> SSQIRQNYSTEVEAAVNRLVNLYLRASYTYLSLGFYFDRDDVALEGVCHFFRELAEEKREGAERLLKMQNQRGGRALF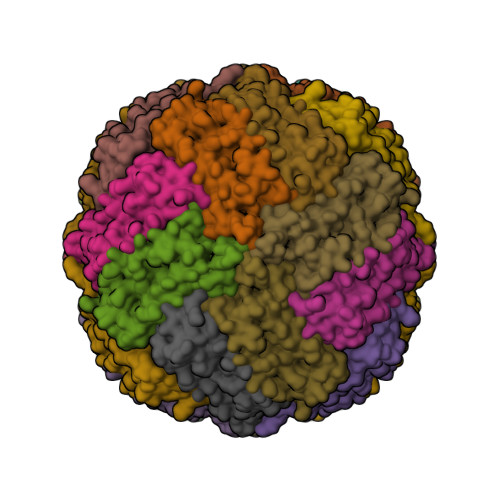QDLQKPSQDEWGTTLDAMKAAIVLEKSLNQALLDLHALGSAQADPHLCDFLESHFLDEEVKLIKKMGDHLTNIQRLVGSQAGLGEYLFERLTLKH> MDKDEAWKQVEQLRREGATQIAYRSDDWRDLKEAWKKGADILIVDATDKDEAWKQVEQLRREGATQIAYRSDDWRDLKEAWKKGADILIVSEEMARHAPKDEAWKQVEQLRREGATQIAYRSDDWRDLKEAWKKGADILIVDATDKDEAWKQVEQLRREGATQIAYRSDDWRDLKEAW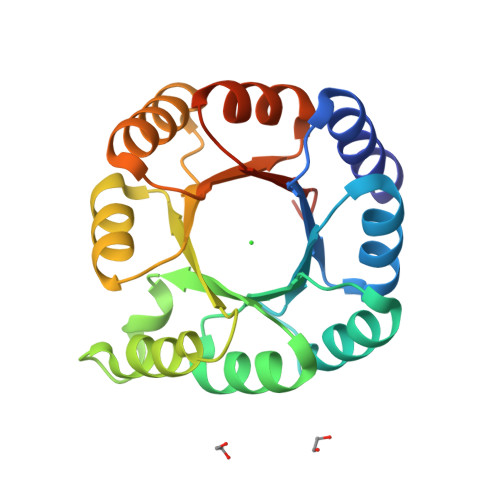KKGADILIVDATGLEHHHHHH> TIDTCSSDSPLSCQTDNEASCCFNSPGGSLLQTQFWDYDPSDGPSDSWTIH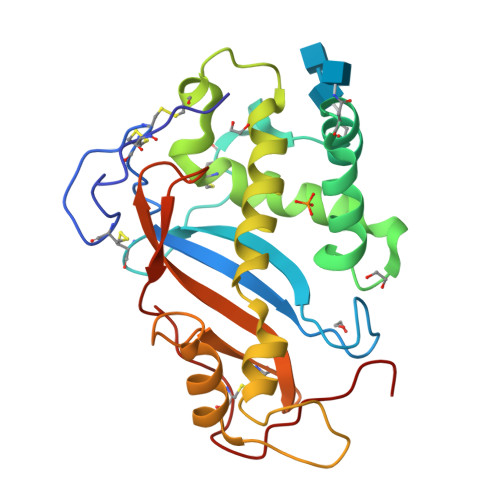GLWPDNCDGTYQEYCDESREYSNITSILEAQNRTELLSYMKEYWPDYEGADEDESFWEHEWNKHGTCINTIEPSCYTDYYAQEEVGDFFQQVVDLFKTLDSYTALSDAGITPSEDATYKLSDIEDALAAIHDGYPPYVGCEDGALSQLYYYFNVKGSAIGGTYVASERLEDSNCKDSGIKYPPKYS>SAFPIDLRGQTAFVAGVADSHGY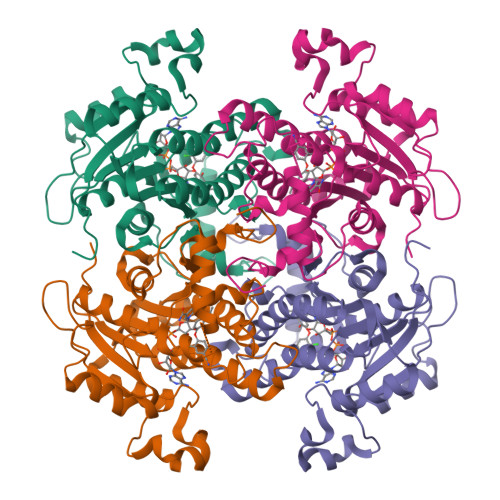GWAIAKHLASAGARVALGTWPPVLGLFQKSLQSGRLDEDRKLPDGSLIEFAGVYPLDAAFDKPEDVPQDIKDNKRYAGVDGYTIKEVAVKVKQDLGNIDILVHSLANGPEVTKPLLETSRKGYLAASSNSAYSFVSLLQHFGPIMNEGGSAVTLSYLAAERVVPGYGGGMSSAKAALESDTRTLAWEAGQKYGVRVNAISAGPLKSRAASAIGKSGEKSFIDYAIDYSYNNAPLRRDLHSDDVGGAALFLLSPLARAVSGVTLYVDNGLHAMGQAVDSRSMPPLQRATQEIN[2x]>[2x]MNIISTSVFVGPNTFARTPLIRLTVDIDPHYAEKLNTLGSEVYQALDQVVPGMSSDPVEQAPGMLIARLALKLQHLAGMEGGIAFTSTSQADDEAEVLYSYETEDIGLEAGEVACDMLVALARAEADVRAVDLSHHIARYLRYADKRTLGPSAMELVKAAQERDIPWYRMNDASLIQVGQGKYQKRIEAALTSKTSHIAVEIAADKNMCNQLLGDLGLPVPKQRVVYDEDEAVSAANRIGYPVVVKPLDGNHGRGVSVSLTDEQAVKKAYGLAEPEGSAVIVESMIRGDDHRLLVVNGELVAAARRVPGHVAGDGIHTIRELIALVNQDPRRGVGHENVLTRLELDEQAIRLLQSYGY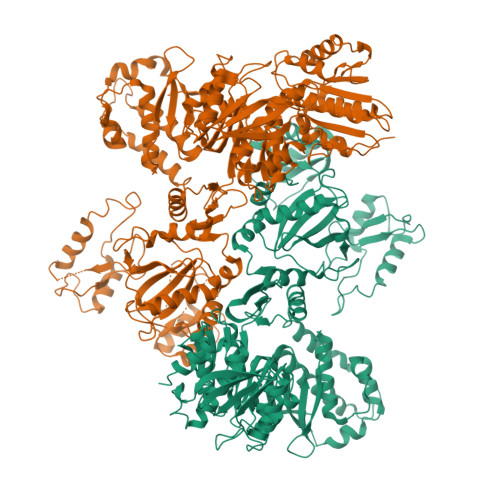TADSIPPSGEEVYLRKTANISTGGTAVDVTDVIHPDNKLMAERAILAVGLDVGAVDFLTTDITKSYRETLGAICEINAGPGLRMHISPSEGKPRDVGGKIMDMLFPAGSQCRVPIAALTGTNGKTTCARMLSHILKMAGHVVGQTSTDAVLIDGNVTVKGDMTGPVSAKMVLRDPSVDIAVLETARGGIVRSGLGYMFCDVGAVLNVTSDHLGLGGVDTLDELAKVKRVIAEVTRDTVVLNADNEYTLKMAAHSPAKHIMYVTRNPEHTLVREHIRLGKRAVVLEQGLNGEQIVIYDNGMQIPLTWTHLIPATLEGKALHNVENAMFAAGMAYALGKTLDQIRSGLRTFDNTFFQSPGRMNVFDGHGFRVILDYGHNEAAIGAMVELVGRLNPQGRRLVAVTCPGDRRDEDVAAIAAKVAGHFDSYICHRDDDLRDRGPDEMPRLMKQALMDRGVKEEAIQIVEQEVDALSTLLKMANRNDLVLFFCENITRCWKQIINFKPAFGEALPAAAPEVLPVQTTDIPAGYQITQGERGVLIIPNDAAAENLYFQ> LAAKEAKLRDLE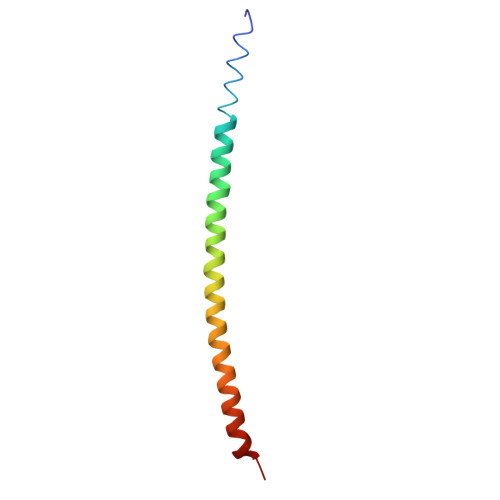DSLARERDTSRRLLAEKEREMAEMRARMQQQLDEYQELLDIKLALDMEIHAYRKLLEGEEER>[2x]GGRMQLTADQVEKYKSDGYVLLEGAFSPEEVHVMRQALKKDQEVQGPHRILEEDGRTVRALYASHTRQSVFDQLSRSDRLLGPATQLLECDLYIHQFKINTKRAFGGDSWAWHQDFIVWRDTDGLPAPRAVNVGVFLSDVTEFNGPVVFLSGSHQRGTVERKARETSRSDQHVDPDDYSMTPAELSQMVEKHPMVSPKAASGSVMLFHPEIIHGSAPNISPFARDLLIITYNDVANAPKPAGEPRPEYVIGRDTTPLVSRSGPLHEAA

Like LdoA and EcdK, GriE belongs to the 2OG-Fe(ii) oxygenase superfamily, whose members couple the decarboxylation of α-ketoglutarate to substrate oxygenation/hydroxylation via an oxo-ferryl intermediate. Recombinant GriH purified from S. lividans TK24 lacked the characteristic fluorescence of the expected F420 co-factor but nevertheless led to 4-MePro in a coupled assay with GriF, indicating that GriH can use NADH directly without requiring F420. Together, these experiments suggest that 4-MePro biosynthesis starts with the GriE-mediated hydroxylation of l-leucine, followed by oxidation with GriF. The crystal structures of the leucine hydroxylase GriE have been determined in complex with substrates and products, providing insight into the stereospecificity of the reaction.

The canonical iron-binding motif is formed by His110, Asp112 and His210 and has lost the metal in the apo structure. While the residues 159–176 were not visible in the electron density of the apo structure, this region is well defined in the ligand complexes. A third loop comprising residues 232–247 is tilted away from the active site in the ligand complexes.>MVSLPRMVYPQPKVLTPCRKDVLVVTPWLAPIVWEGTFNIDILNEQFRLQNTTIGLTVFAI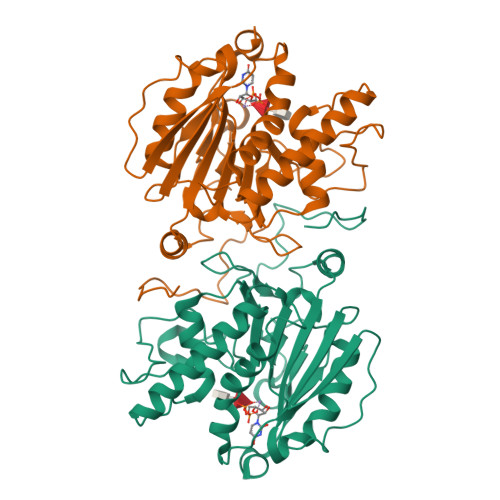KKYVAFLKLFLETAEKHFMVGHRVHYYVFTDQLAAVPRVTLGTGRQLSVLEVRAYKRWQDVSMRRMEMISDFCERRFLSEVDYLVCVDVDMEFRDHVGVEILTPLFGTLHPGFYGSSREAFTYERRPQSQAYIPKDEGDFYYLGGFFGGSVQEVQRLTRACHQAMMVDQANGIEAVWHDESHLNKYLLRHKPTKVLSPEYLWDQQLLGWPAVLRKLRFTAVPKNHQAVRNP[2x]>[2x]MMISEVKQDAKSRMEKSLSVYLSDIDGIRTGRARTSVLNGIVVETYGGRVKLNTISSVSVSDNKTLMIKVWDSNNIGAIKTAIMNSNLGFGISCEATTIRLTVPDMTQDMRKNLVKLLGKI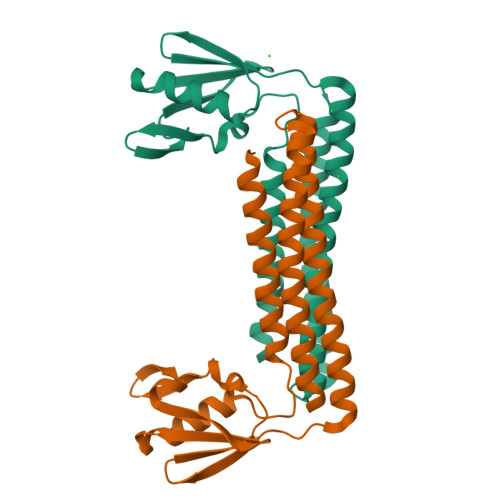SEDCRVSIRNIRRDIMDRLKVMQDSKEISEDDLRVAGVEIQKITDDIMKKVNDAFTSKEKELLHVGHHHHHH> MLKQVEIFTDGSALGNPGPGGYGAILRYRGREKTFSAGYTRTTNNRMELMAAIV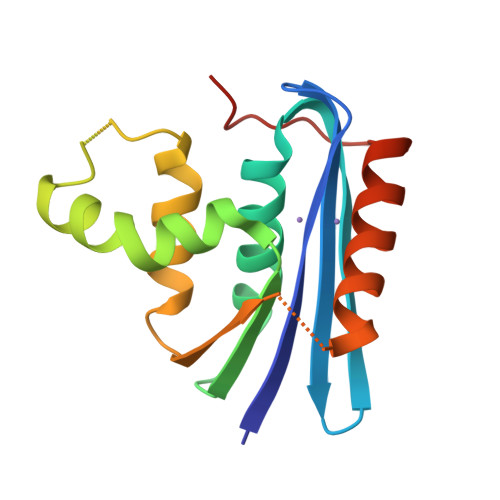ALEALKEHAEVILSTDSQYVRQGITQWIHNWKARGWKTADKKPVKNVDLWQRLDAALGQHQIKWEWVKGHAGHPENERADELARAAAMNPTLEDTGYQVEV> MVDFKTYFELLNLY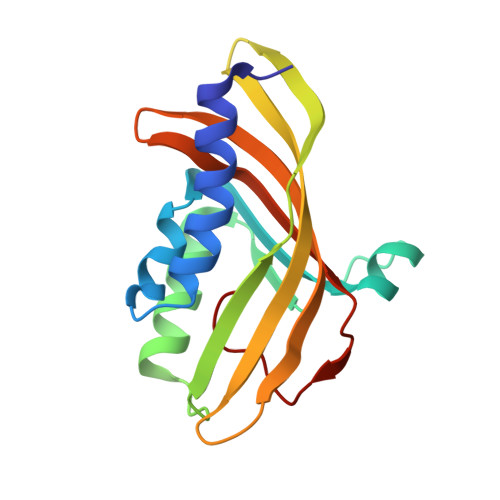SDYAMVCDSANWEKWPDFFIETGTYRLQPRENFEQGLPLCLLALESKAMIRDRVYGVKETMYHDPYYQRHIVGTPRVLSVERDADGERITAEASYAVIRTKYDGDSTIFNAGYYRDVIVRTPEGLKLKSRLCVYDSEMIPNSVIYPI>[2x]MIEAPDVKPWLFLIKPYEGESLSHFLGRFRRANHLSASGLGTLAGIGAIVARWERFHFNPRPSQQELEAIASVVEVDAQRLAQMLPPAGVGMQHEP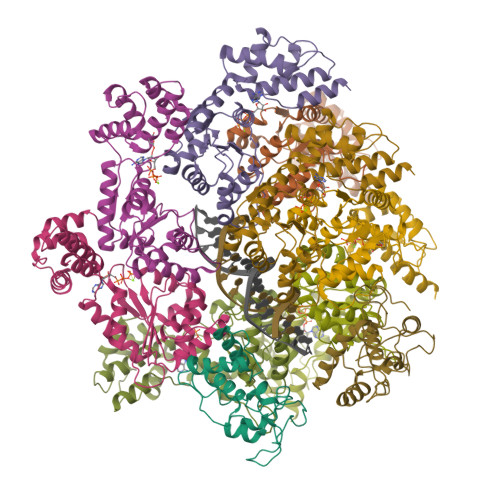IRLCGACYAESPCHRIEWQYKSVWKCDRHQLKILAKCPNCQAPFKMPALWEDGCCHRCRMPFAEMAKLQKV;>MTEAQAIAKQLGGVKPDDEWLQAEIARLKGKSIVPLQQVKTLHDWLDGKRKARKSCRVVGESRTGKTVACDAYRYRHKPQQEAGRPPTVPVVYIRPHQKCGPKDLFKKITEYLKYRVTKGTVSDFRDRTIEVLKGCGVEMLIIDEADRLKPETFADVRDIAEDLGIAVVLVGTDRLDAVIKRDEQVLERFRAHLRFGKLSGEDFKNTVEMWEQMVLKLPVSSNLKSKEMLRILTSATEGYIGRLDEILREAAIRSLSRGLKKIDKAVLQEVAKEYK[8x]[2-[(4-oxidanylidene-3,5-dihydropyrrolo[3,2-d]pyrimidin-7-yl)sulfanyl]phenoxy]methylphosphonic 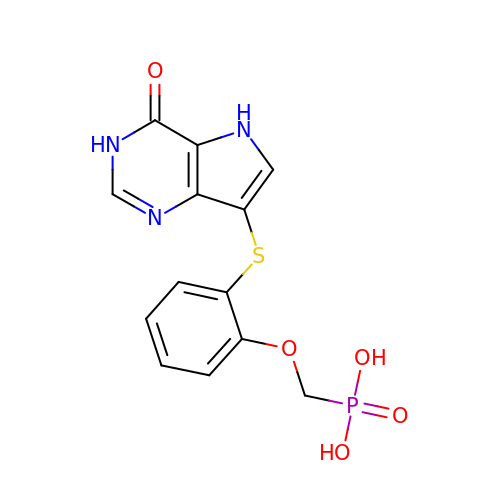acid | C13 H12 N3 O5 P S | VOAJLIGXNWIOPN-UHFFFAOYSA-N> ECCSRGDAEVVISEWDQVFNAAMAGSSESAVGVAIFDAFFASSGVSPSMFPGGGDSNNPEFLAQVSRVVSGADIAINSLTNRATC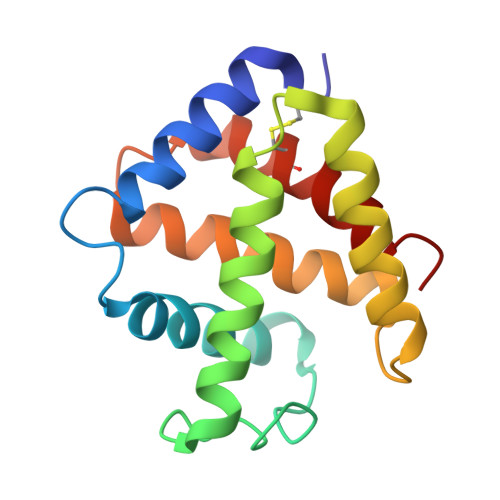DSLLSHLNAQHRAISGVTGAAVTHLSQAISSVVAQVLPSAHIDAWEYCMAYIAAGIGAGL>GMISDSISKRRSIRKYKNQSISHETIEKIIEAGINAPSSKNRQPWRFVVITEKEKESMLKAMSKGIQNEINDNGLLPGSRQHIAGANYTVEIMKQAPVTIFILNILGKSPLEKLSPEERFYEMANMQSIGAAIQNMSLTAVELGLGSLWICDVYF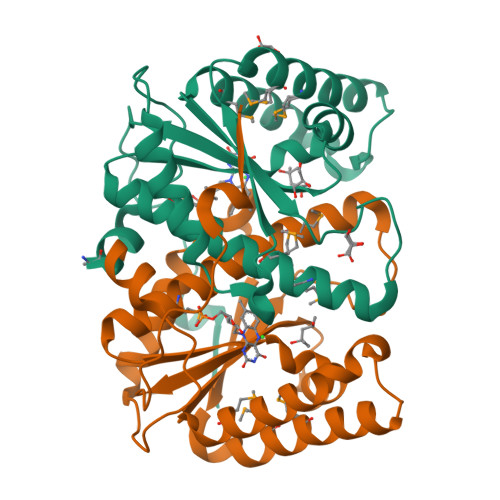AYRELCEWLNTDSQLVAAISLGYPDEEPSRRPRLQLSDVTEWR[2x]>[3x]HHHHHHSSGLVPRGSHMRSGTMDRMPPRPSTRDQRSSGDSRGGRWSPRLTVFD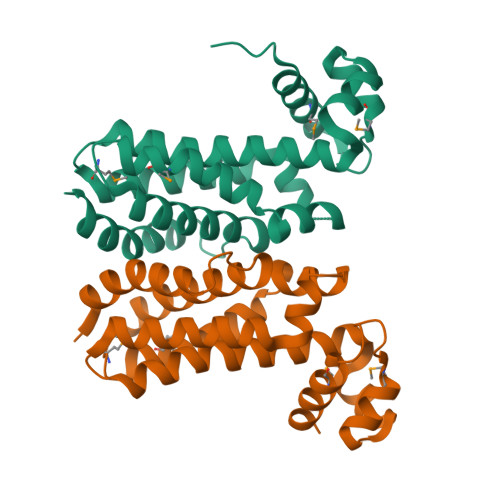AMHQLLESRDWSAVTMSDVAKAAGLSRQTLYSTFGNRQGLAQAYALQLSEKFAGEIRDSIIRHPGQIELALSEGINGFLRSSSRDPLIRALVTGDIKPDLLRLITTEAGPLIERATEVLMPALSESWMRIEASQARLAASIIARIGISFISLPPEDPDQLASGLTEVIAPYLQKVVQVDVQQ>GSHMLRISQEALTFDDVLLIPGYSEVLPKDVSLKTRLTRGIELNIPLVSAAMDTVTEARLAIAMAQEGGIGIIHKNMGIEQQAAEVRKVKKHETAIVRDPVTVTPSTKIIELLQMAREYGFSGFPVVEQGELVGIVTGRDLRVKPNAGDTVAAIMTPKDKLVTAREGTPLEEMKAKLYENRIEKMLVVDENFYLRGLVTFRDIEKAKTYPLASKDEQGRLRVGAAVGTGADTGERVAALVAAGVDVVVVDTAHGHSKGVIERVRWVKQTFPDVQVIGGNIATAEAAKALAEAGADAVKVGIGPGSICTTRIVAGVGVPQISAIANVAAALEGTGVPLIADGGIRFSGDLAKAMVAGAYCVMMGSMFAGTEEAPGEIELFQGRSYKSYRGMGSLGAMSGSQGSSDRYFQDASAGAEKLVPEGIEGRVPYKGALSAIVHQLMGGLRAAMGYTGSADIQQMRTQPQFVRITGAGMAESHVHDVQITKEAPNYRVG[2x]

IMP dehydrogenase (IMPDH) catalyzes the first step in the guanine nucleotide de novo biosynthetic pathway, at the bifurcation of the guanine and adenine routes, which share the precursor IMP. An IMPDH monomer consists of a catalytic TIM barrel (light blue) and a regulatory Bateman domain (dark blue), which is not required for catalytic activity but is essential for allosteric regulation. The basic units of IMPDH are tetramers that dimerize to form octamers upon nucleotide binding. In contrast to the eukaryotic enzymes, bacterial IMPDHs only contains two canonical allosteric binding sites in their Bateman domains.

After multiple cocrystallization trials, we were able to obtain the structure of PaIMPDH bound to both ATP and GDP at 1.65 Å resolution (Table SS1). The two monomers in the asymmetric unit (AU) contained well‐defined electron density in the Bateman domain that could be unequivocally attributed to ATP and GDP bound to the canonical Sites 1 and 2, respectively, as well as a magnesium atom coordinated by their β‐ and γ‐phosphates. The binding modes of ATP and GDP in the canonical sites are identical to those observed in the structures of eukaryotic IMPDHs, 6 , 13 , 14 , 34 where the nucleotide's phosphate groups position close together at the interface of two opposing Bateman domains. The recognition of the adenine ring of ATP bound to the canonical Site 1 (ATP1) was mainly due to hydrogen bonds from the backbone carbonyl atoms of residues V159 and K181 and N6 nitrogen atom of the adenine. Additionally, ATP1 γ‐phosphate coordinated a Magnesium atom, together with the β‐phosphate of GDP bound to the canonical Site 2 (GDP2) and the carboxylic acid in the side chain of residue E180. In the canonical Site 2, GDP2 guanine ring was sandwiched between the hydrophobic side chains of residues F118 and V94, with the hydroxyls of the ribose moiety tightly coordinated to the carboxylic acid of the absolutely conserved residue D199. 35 The negative charge of GDP2 phosphate groups was counteracted by the basic side chains of residues K181 and R198, as well as a Magnesium atom. Monomers in the AU are related by noncrystallographic symmetry axes that allow to reconstruct IMPDH octamers within the crystal lattice. These octamers are assembled as dimers of tetramers that pile up tail‐to‐tail, forcing the finger domains of opposing tetramers to interact and placing their catalytic sites close together to inhibit the catalytic activity. Remarkably, no electron density surrounding the area corresponding to the eukaryotic noncanonical Site 3 is observed in the inhibited PaIMPDH structure, suggesting that, in contrast to eukaryotic IMPDHs, the occupancy of the canonical Site 2 by GTP/GDP (when ATP is bound at the canonical Site 1) is necessary and sufficient to induce compact octamers and, subsequently, inhibit the activity of PaIMPDH and EcIMPDH.> MDNNYHFWGNGDRQDVSLSYEDYYSILDCLLDEKLSPQGLMKFKNLHEVSMYGVSYVPLYCFPVAYGISHMLTGKVR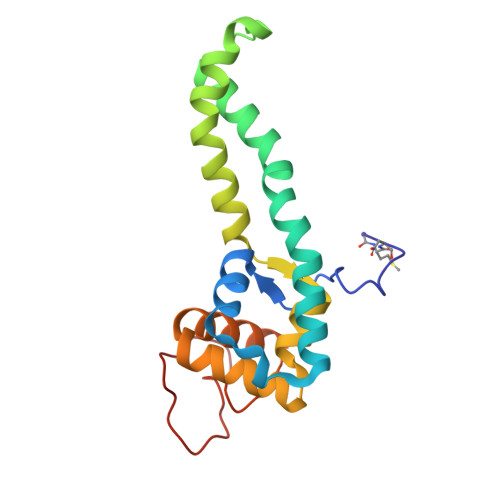RGHSGYRNLFSLMSVVLPFTCWYAYTTPIPRRLYTEIICSNNADGAYVRNRIKQQKPGIWRKLSQQLYNKNFRFPELNQDLTATEFPLDYVAPHKF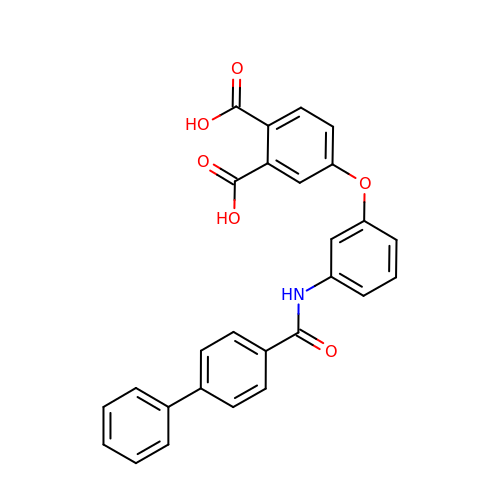4-{3-[(biphenyl-4-ylcarbonyl)amino]phenoxy}benzene-1,2-dicarboxylic acid | C27 H19 N O6 | RUUIIXBPIYJULM-UHFFFAOYSA-N>[4x]RRKKPQDHFFDVPA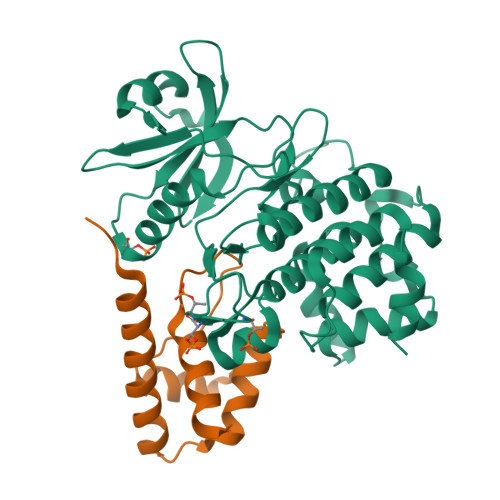EEDPEVHLGQLKRFSLRELQVASDNFSNKNILGRGGFGKVYKGRLADGTLVAVKRLKEERTQGGELQFQTEVEMISMAVHRNLLRLRGFCMTPTERLLVYPYMANGSVASCLRERPESQPPLDWPKRQRIALGSARGLAYLHDHCDPKIIHRDVKAANILLDEEFEAVVGDFGLAKLMDYKDTHVTTAVRGTIGHIAPEYLSTGKSSEKTDVFGYGVMLLELITGQRAFDLARLANDDDVMLLDWVKGLLKEKKLEALVDVDLQGNYKDEEVEQLIQVALLCTQSSPMERPKMSEVVRMLEGDGLAERWEEWQKEEMFRQDFNYPTHLEHHHHHH;>GPLGSDRASQTPVDRSPPRVNQRPIRVDRAAMRNRGNDEADAALRGLVQQGVNLEHLRTALERHVMQRLPIPLDIGSALQNVGINPSIDLGESLVQHPLLNLNVALNRMLGLRPSAE[4x]>MIRGSSALKSLTSRRLYSTGVKYTTLSNGVTVATETNPAAKTSSVGLFFGAGSRSEHSHSNGISALTTNVLASQSAKGSLLTAKNDREFNGIIAQTTNDNITEAGKLIASIASNAVDIVEKTDLTKHKQYLSAQASAVEADPKSKVLSHLYSSAFQGYSLALPTLGTTESVENLENQDSLRHLAKHLVNNNTVIAASGNFDHDKLADAIEANLKIAEGVKPEIKPASFLGSEVRMRDDTLPKAYISIAVHGEGLNSPNYYLAKVAAAIYGDFYLHSTIAKFTSPKLASIVQEYNIVESYNHYSKSFSDTGIWGYYAEIADKFTVDDFTHFSLKEWNRLSISISEAEVARAKAQVKTALAKELANSFAVTSDIAEKVLLVGHRQSLREAFEKIDAIKVNDVKEWGKSKVWDRDIVISGTGLIEDLLDYNRNRNEMAMMRW[2x];>[2x]MLSRASIRAYSSIPNSVKIAAKESATDLTKLSVIINNAGSKTGKSGVSHLLSKFTFLNNGAKSALRFTRESELLGGTFESKVTRDALILNTTFLKQDLPYYVEALGNVVSNTQFAPHEFNEIVLPTANAETKLANANPAFKGVEKLHEITFRRGLGNPLFYNESTPIKLEEVAQFSKEQFSGENISIVAEGANEEDLTKFVSESAFCYLPSSSSNGAKALPTNTFTGQEARVPSSGASSALIGIPVKPADFGKYEVLSAAIGTSTLPSTSTPLAQIPGATSHLYKYQDAGLFVISVSGEASQVAQGIKQAKSVAESVSSSALSEAVKAAELSVALQSTVDSPLNVKVVAEEAPISKFNYVAVGDLDVLPYADEL;>[2x]MSSLAFRTLRNGLGLKSSVRALSTTTTTLSNYQQPDYSSYLNNKSGQGSRNFTYFMVGSMGLLSAAGAKSTVEAFLSSFAASADVLAMAKVEVKLGAIPEGKNVIIKWQGKPVFIRHRTADEIEEANQVDIKTLRDPQNDADRVKKPEWLIMLGICTHLGCVPIGEAGDFGGWFCPCHGSHYDISGRIRKGPAPLNLEIPEYDFTDDETLLVG;>[2x]MFRTAYKTMNQSMVQKFIAGGVGVTGLTASYLLYQDSMTADAMTAAEHGLHPPAYNWPHNGMFETFDHASIRRGFQVYREVCAACHSLDRIAWRNLVGVSHTTSEAKAMAEELEYDDEPDDEGKPRKRPGKLADYIPGPYENEQAARAANQGAYPPDLSLIVKARHGGSDYIFSLLTGYPDEPPAGVVLPEGSNYNPYFPGGAIAMGRVLFDDLVEYEDGTPATTSQMAKDVSTFLNWASEPEHDDRKKWGLKALVVLSSLYLLSIWVKRFKWTPIKNRKFRFDPPKK;>[2x]MAGAPHPHTYMGWWGSLGSPKQKYITQYTISPYAAKPLKGAAYNAVFNTFRRTKNQFLYVAIPFVVVWSIWTRARDYNEYLYTKEGREELERVNV;>MVQSMTSVVKAANFILARPTLSKIITPLAQKFTAYAGYREMGLKFNDLLLEETPIMQTAIKRLPSELNYSRNFRILTAHQLALSHQLLPAEKAVKPEEDDNYLIPYILEAEKEAFEKAELDNIEVKA[2x];>MSFFRDLLESVVPTAYAEEPVEDVEVEQPEDAPEEEVSEETVEEEEEDDEDDDEDDEEEEETADPLDTLREECTKTAACKPFDHHFHECIERVTKEQEEPDYEHKHYKEDCIEEFFHLQHCVNDCVAPRLFNRLK[2x];>MLTVLGRLLERNSIYVATIFGGAFAFQGFFDVAVNKWWEEHNKAKLWKNVKGKFLEGEGEEEDDE[2x];>MPTRKSNTYLSLVNSYLIDSPQPSSINYWWNLGSLLGLCLVIQIASGVFLAMHYSSNIELAFDSVEHIMRDVNAGWLIRYIHANGASFFFICMYLHIGKALYYGSYKQPRVMLWVIGVVIFILTMAIAFMGYCLVYGQMSHWGATVITNLLSAIPFIGNDIVPFIWGGFSVSNPTIQRFFALHFLLPFILAALVCMHLMALHVHGSSNPVGITGNIDRLPMHPYFIFKDLITVFVFLLIFSLFVFYSPNTLGHPDNYIPGNPMVTPPSIVPEWYLLPFYAILRSIPDKLGGVIAMFGAILILLSLPYTDRSIIRGNSFKVLSKLAFYLFVFNFILLGNLGQLHVEVPYIQLGQFATAYYFAHYIIVVPVISTLE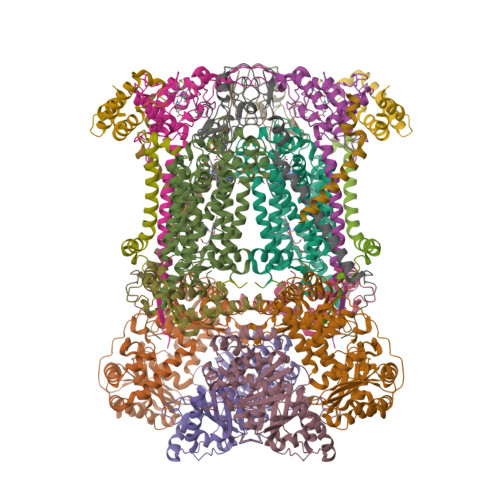NILYYIGTQTRVK[2x]>MPRGSRSAASRPASLPAA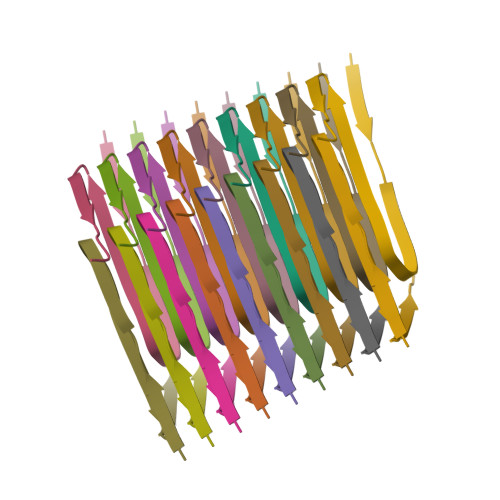PSAHPPAHPPPSAAAPAPAPSGQPGLMAQMATTAAGVAVGSAVGHVMGSALTGAFSGGSSEPSQPAVQQAPTPAAPQPLQ[18x]> MQQQCDTVSAWQSLRGPGTGGYYLFKTTEGGKTDCTYVKGSNFNDAAQTATYTYGNLGSGNQLTQQTASASISGNAIVVGTDHSEVLYSDGSTCDVVRLNGQIELWIHSSATSNTGNLNSCCTDKFNQEK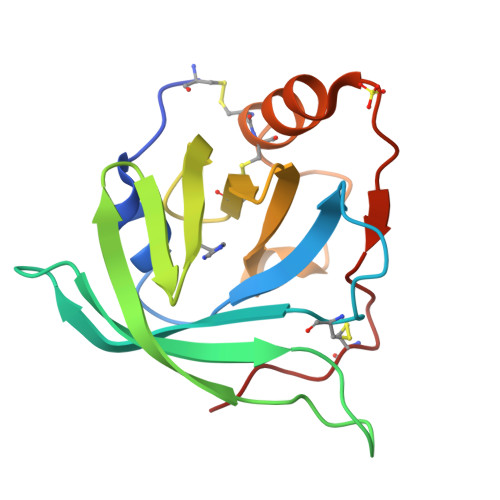GSRPEHVVYRSTCPNLPQ8-AMINO-1,3-DIMETHYL-3,7-DIHYDROPURINE-2,6-DIONE | C7 H9 N5 O2 | 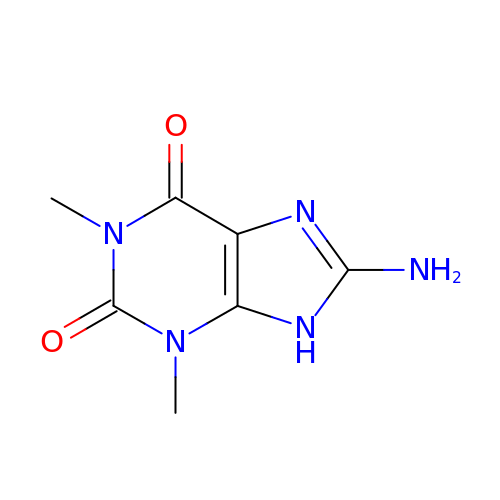ZZESAIGPDOBLKZ-UHFFFAOYSA-N> RRIGEIVKVVQAAARGWVERKHFRQAREKSVSARIIQDNIRAYLEFKNWAWWKLFAKARPLLV;> TASADQIQECF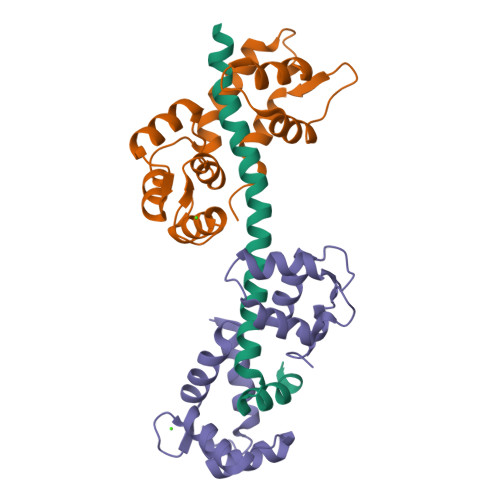QIFDKDNDGKVSIEELGSALRSLGKNPTNAELNTIKGQLNAKEFDLATFKTVYRKPIKTPTEQSKEMLDAFRALDKEGNGTIQEAELRQLLLNLGDALTSSEVEELMKEVSVSGDGAINYESFVDMLVTGYPLA;> GDDQVSEFKEAFELFDSERTGFITKEGLQTVLKQFGVRVEPAAFNEMFNEADATGNGKIQFPEFLSMMGRRMKQTTSEDILRQAFRTFDPEGTGYIPKAALQDALLNLGDRLKPHEFAEFLGITETEKGQIRYDNFINTMFT>[12x]QTIEENIKIFEEEEVEFISVPV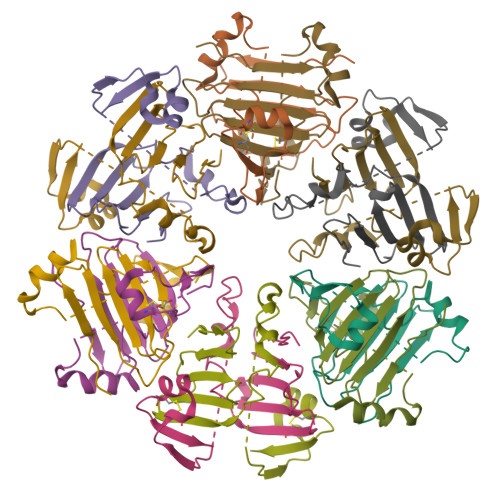PEFADSDPANIVHDFNKKLTAYLDLNLDKCYVIPLNTSIVMPPRNLLELLINIKAGTYLPQSYLIHEHMVITDRIENIDHLGFFIYRLCHDKETYKL>[2x]MESRVTPVAVIGMGCRLPGGINSPDKLWESLLRGDDLVTEIPPDRWDADDYYDPEPGVPGRSVSRWGGFLDDVAGFDAEFFGISEREATSIDPQQRLLLETSWEAIEHAGLDPASLAGSSTAVFTGLTHEDYLVLTTTAGGLASPYVVTGLNNSVASGRIAHTLGLHGPAMTFDTACSSGLMAVHLACRSLHDGEADLALAGGCAVLLEPHASVAASAQGMLSSTGRCHSFDADADGFVRSEGCAMVLLKRLPDALRDGNRIFAVVRGTATNQDGRTETLTMPSEDAQVAVYRAALAAAGVQPETVGVVEAHGTGTPIGDPIEYRSLARVYGAGTPCALGSAKSNMGHSTASAGTVGLIKAILSLRHGVVPPLLHFNRLPDELSDVETGLFVPQAVTPWPNGNDHTPKRVAVSSFGMSGTNVHAIVEEAPAEASAPESSPGDAEVGPRLFMLSSTSSDALRQTARQLATWVEEHQDCVAASDLAYTLARGRAHRPVRTAVVAANLPELVEGLREVADGDALYDAAVGHGDRGPVWVFSGQGSQWAAMGTQLLASEPVFAATIAKLEPVIAAESGFSVTEAITAQQTVTGIDKVQPAVFAVQVALAATMEQTYGVRPGAVVGHSMGESAAAVVAGALSLEDAARVICRRSKLMTRIAGAGAMGSVELPAKQVNSELMARGIDDVVVSVVASPQSTVIGGTSDTVRDLIARWEQRDVMAREVAVDVASHSPQVDPILDDLAAALADIAPMTPKVPYYSATLFDPREQPVCDGAYWVDNLRNTVQFAAAVQAAMEDGYRVFAELSPHPLLTHAVEQTGRSLDMSVAALAGMRREQPLPHGLRGLLTELHRAGAALDYSALYPAGRLVDAPLPAWTHARLFIDDDGQEQRAQGACTITVHPLLGSHVRLTEEPERHVWQGDVGTSVLSWLSDHQVHNVAALPGAAYCEMALAAAAEVFGEAAEVRDITFEQMLLLDEQTPIDAVASIDAPGVVNFTVETNRDGETTRHATAALRAAEDDCPPPGYDITALLQAHPHAVNGTAMRESFAERGVTLGAAFGGLTTAHTAEAGAATVLAEVALPASIRFQQGAYRIHPALLDACFQSVGAGVQAGTATGGLLLPLGVRSLRAYGPTRNARYCYTRLTKAFNDGTRGGEADLDVLDQHGTVLLAVRGLRMGTGTSERDERDRLVSERLLTLGWQQRALPEVGDGEAGSWLLIDTSNAVDTPDMLASTLTDALKSHGPQGTECASLSWSVQDTPPNDQAGLEKLGSQLRGRDGVVIVYGPRVGDPDEHSLLAGREQVRHLVRITRELAEFEGELPRLFVVTRQAQIVKPHDSGERANLEQAGLRGLLRVISSEHPMLRTTLIDVDEHTDVERVAQQLLSGSEEDETAWRNGDWYVARLTPSPLGHEERRTAVLDPDHDGMRVQVRRPGDLQTLEFVASDRVPPGPGQIEVAVSMSSINFADVLIAFGRFPIIDDREPQLGMDFVGVVTAVGEGVTGHQVGDRVGGFSEGGCWRTFLTCDANLAVTLPPGLTDEQAITAATAHATAWYGLNDLAQIKAGDKVLIHSATGGVGQAAISIARAKGAEIFATAGNPAKRAMLRDMGVEHVYDSRSVEFAEQIRRDTDGYGVDIVLNSLTGAAQRAGLELLAFGGRFVEIGKADVYGNTRLGLFPFRRGLTFYYLDLALMSVTQPDRVRELLATVFKLTADGVLTAPQCTHYPLAEAA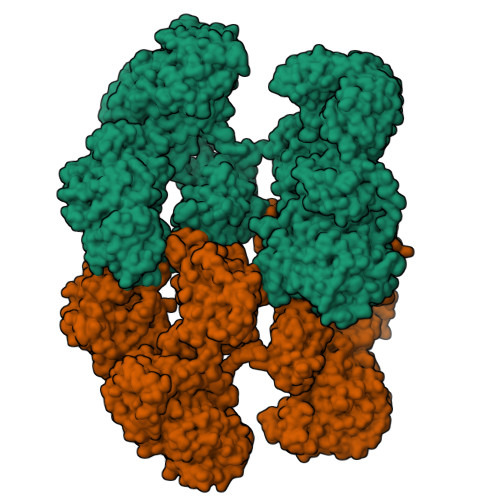DAIRAMSNAEHTGKLVLDVPRSGRRSVAVTPEQAPLYRRDGSYIITGGLGGLGLFFASKLAAAGCGRIVLTARSQPNPKARQTIEGLRAAGADIVVECGNIAEPDTADRLVSAATATGLPLRGVLHSAAVVEDATLTNITDELIDRDWSPKVFGSWNLHRATLGQPLDWFCLFSSGAALLGSPGQGAYAAANSWVDVFAHWRRAQGLPVSAIAWGAWGEVGRATFLAEGGEIMITPEEGAYAFETLVRHDRAYSGYIPILGAPWLADLVRRSPWGEMFASTGQRSRGPSKFRMELLSLPQDEWAGRLRRLLVEQASVILRRTIDADRSFIEYGLDSLGMLEMRTHVETETGIRLTPKVIATNNTARALAQYLADTLAEEQAAAPAASKLAAALEHHHHHH>[4x]MTDVAKTLEELATERGMRMTEQRRVIARILEDSEDHPDVEELYRRSVKVDAKISISTVYRTVKLF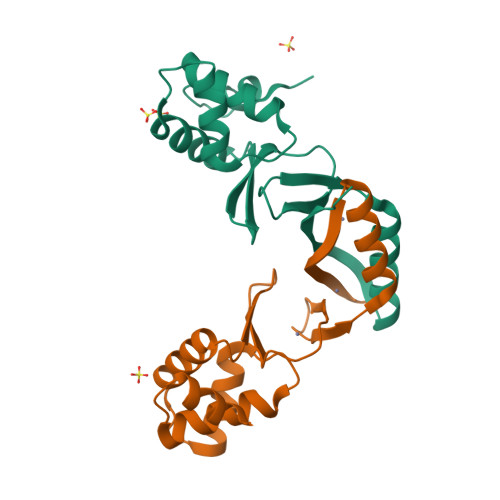EDAGIIARHDFRDGRSRYETVPEEHHDHLIDLKTGTVIEFRSPEIEALQERIAREHGFRLVDHRLELYGVPLKKEDL> MSLIGEILPLSHIVLDMEVGSKKRLFEEAGLLLERESSLSHADVFECLFA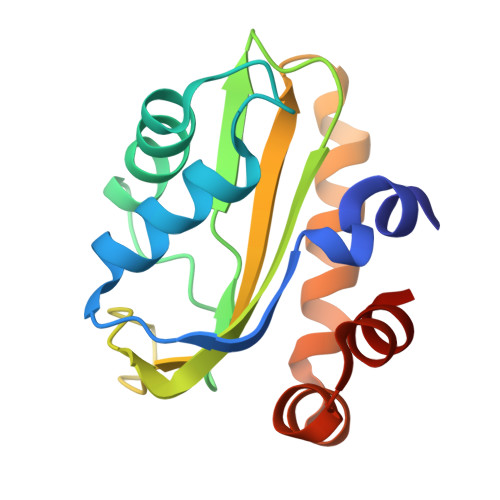REKLGSTGLGQGVAIPHGRHAGVKQATGAFIRTREPVGFDAPDGKPVSLIFILLVPENATGEHLEVLSKLAGKFSQKSIRESLMTVSSAEEVRAILTEE> KKSFFDKK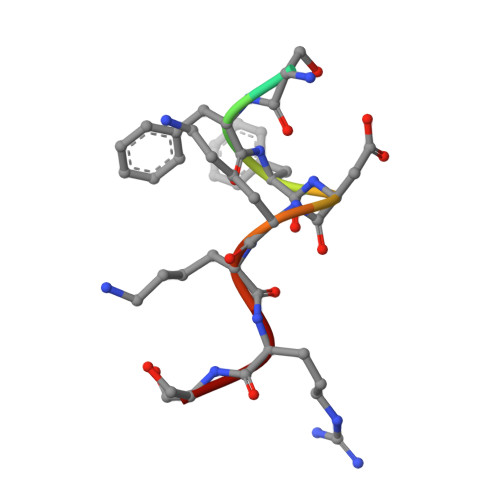RS> SKGENSKLNPWAVVGFIDAEGSFMVRVRKNSKYKTGWLVVAIFSVTVDKKDLFLLESLKTFFGGLGSIKKSGNSTFSYRIESSEQLTKIILPFFDKYSLITEALGDYLLFKKVLELMGTKEHLTQRGLEKIVSLKASINKGLSEELQAAFPQC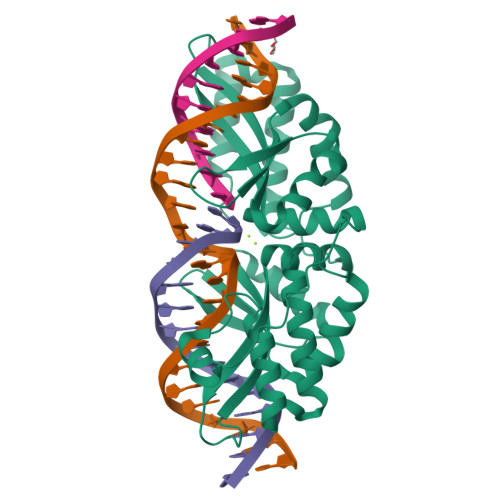VPTPRPEINNKNIPDPFWLAGFVSGDGSFKSILKKSESIKVGFQSILVFQITQHARDVKLMESLISYLGCGFIEKDSRGPWLYYTVTNFSDIQGKIIPFFHQYKIIGSKYGDYQDWCKIALIMQNKNHLTPEGLNEIRALKGGMNKGRL>MILDVDYITEEGKPVIRLFKKENGKFKIEHDRTFRPYIYALLRDDSKIEEVKKITGERHGKIVRIVDVEKVEKKFLGKPITVWKLYLEHPQDQPTIREKVREHPAVVDIFEYDIPFAKRYLIDKGLIPMEGEEELKILAFAIATLYHEGEEFGKGPIIMISYADENEAKVITWKNIDLPYVEVVSSEREMIKRFLRIIREKDPDIIVTYNGDSFDFPYLAKRAEKLGIKLTIGRDGSEPKMQRIGDMTAVEVKGRIHFDLYHVITRTINLPTYTLEAVYEAIFGKPKEKVYADEIAKAWESGENLERVAKYSMEDAKATYELGKEFLPMEIQLSRLIGQPLWDVSRSSTGNLVEWFLLRKAYERNEVAPNKPSEEEYQRRLRESYTGGFVKEPEKGLWDDIVYLDFIALYPSIIITHNVSPDTLNLEGCKNYDIAPQVGHKFCKDIPGFIPSLLGHLLEERQKIKTKMKETQDPIEKILLDYRQKAIKLLANSFYGYYGYAKARWYCKECAESVTAWGRKYI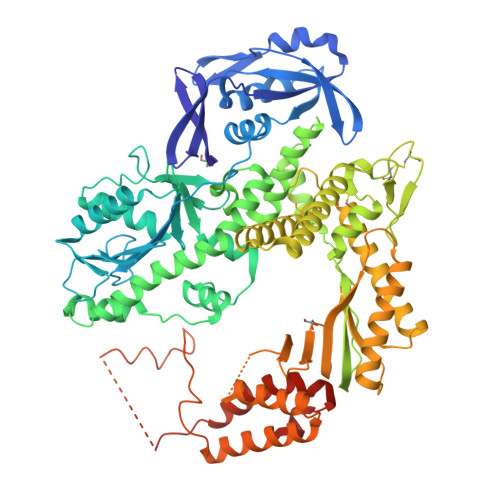ELVWKELEEKFGFKVLYIDTDGLHATIPGGESEEIKKKALEFVKYINSKLPGLLELEYEGFYKRGFFVTKKRYAVIDEEGKVITRGLEIVRRDWSEIAKETQARVLETILKHGDVEEAVRIVKEVIQKLANYEIPPEKLAIYEQITRPLHEYKAIGPHVAVAKKLAAKGVKIKPGMVIGYIVLRGDGPISNRAILAEEYDPKKHKYDAEYYIENQVLPAVLRILEGFGYRKEDLRYQKTRQVGLTSWLNIKKS[2x]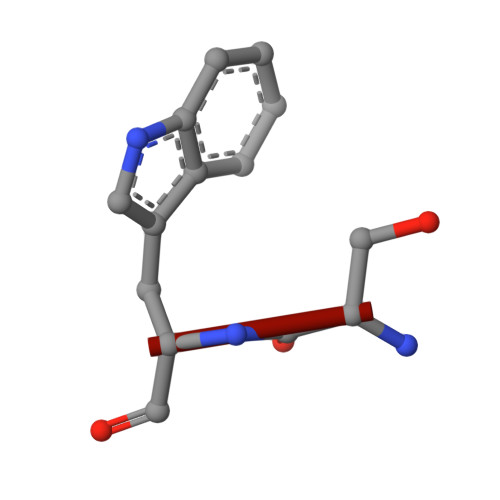> SW> PGAPPGRD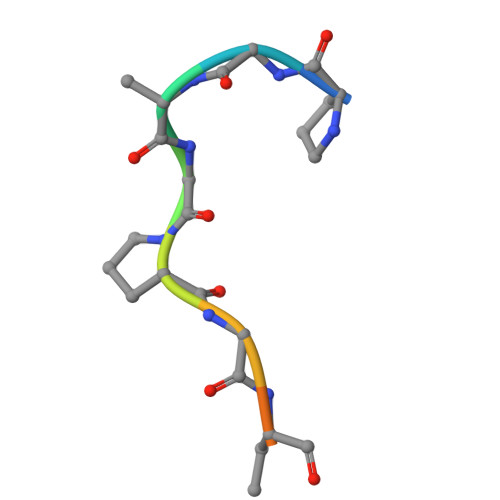LA>MDKIVIAIDAGHGGQDPGAIGPGGTREKNVTIAIARKLRTLLNADPMFKGVLTRDGDYFISVMGRSDVARKQNANFLVSIHADAAPNRSATGASVWVLSNRRANSEMANWLEEHEKQSELLGGAGDVLANSQSDPYLSQAVLDLQFGHSQRVGYDVATNMLGQLERIGSLHKRRPEHASLGVLRSPDIPSVLVETGFISNHGEERLLASDEYQQRLAEAIYQGLRNYFQAHPLQ[2x];> MGSSHHHHHHSQDPMSRTGGLGSPRGQAYWPVRGPTLHRYGEQLQGELRWKGMVIGASEGTEVKAIADGRVILADWLQGYGLVVVVEHGKGDMSLYGYNQSALVSVGTQVRAGQPIALVGSSGGQGRPSLYFEIRRQGQAVNPQPWLGR

Peptidoglycan amidases are key hydrolytic enzymes that are needed to break the peptidoglycan layer during cell division to allow for separation of daughter cells. All the three division-associated amidases have overlapping enzymatic functions in hydrolyzing the peptidoglycan amide bond between the sugar and the first amino acid of the peptide cross-link. In their resting states, zinc-dependent peptidoglycan amidases such as AmiB and AmiC adopt autoinhibited conformations in which their active sites are blocked by an alpha helix containing a conserved glutamate residue which binds to the active-site zinc. The activators share a common motif, the LytM domain, which forms the proposed site of amidase binding and activation.

After extensive crystallization trials, we were ultimately successful in solving a crystal structure of the AmiB hydrolytic domain bound to the EnvC LytM domain using proteins from Citrobacter rodentium. First, the EnvC LytM domain is bound directly to the amidase interaction helix, with the latter’s hydrophobic residues all pointing directly into the LytM groove. Second, the amidase regulatory domain has a very different conformation in the EnvC-bound structure such that the interaction helix is contiguous with helix 5 and the blocking helix is displaced from the active site. Finally, the active-site zinc is ligated by three residues rather than the five due to the absence of the blocking helix glutamate (Glu167 in AmiA) and dissociation of one of the aspartates (Asp271 in AmiB, equivalent to Asp135 in AmiA). The structure of the EnvC–LytM AmiB complex shows that the amidase interaction helix binds within the same groove as the restraining arm, lending further support for this mechanism. Additionally, the activator–amidase structure further identifies a distinctive loop (C. rodentium EnvC residues G319–G330) that contacts residues located between the interaction helix and helix 5. The extended loop wraps around the residues located between the interaction helix and helix 5, causing them to form a single, continuous, helical element. In the EnvC LytM AmiB costructure, the angles between neighboring ligating residues and the zinc are all close to 109°, suggesting a tetrahedral coordination state in which the fourth position remains open for substrate binding and catalysis. Inspecting the density surrounding the zinc, a low-occupancy ligand is present at the fourth position of the coordination sphere.> MLPDEEKLKLLDTLLTMVEWVKELLEESVEKNSRMRH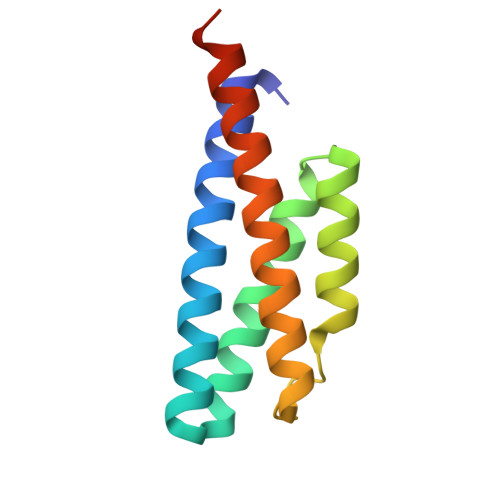IRAVMWAEYMLEIARSLEDEKILEIAEKLEKALPEKSKMFTKEEYEKLMEVLEELEEVLEEKKEEVEERIEGSHHHHH> GHMSQSNRELVVDFLSYKLSQKGYSWSQFSDVEENRTEAPEETEAERETPSAINGNPSWHLADSPAVNGATGHSSSLDAREVIPESAVKQALREAGDEFELRYRRAFSDLTSQLHITPGTAYQSFEQVVNELFRDGVNWGRIVAFFSFGGALCVESVDKEMQVLVSRIASWMATYLNDHLEPWIQENGGWDTFVDLYG;> XIWIAQELRRRGDSFNAYYAR

Another subgroup is composed of antiapoptotic proteins, BCL-2, BCL-XL, BCl-w, MCL-1, A1 and BCL-B, which contain the BH1-BH4 domains that are arranged to form an extended hydrophobic groove known as the BH3-binding groove. The antiapoptotic BCL-2 subfamily proteins bind the BH3 domain of BAX/BAK and of the BH3-only proteins through their BH3-binding groove. Anticancer BH3 peptides have been developed, especially those derived from BIM, which interacts with all of the antiapoptotic proteins with extremely high affinity. Herein, we describe the embedment of the Akt recognition sequence into the BIM BH3 peptide and the cancer cell-specific apoptogenic property of the resulting BIM BH3 peptide variant characterized by X-ray crystallography, calorimetry and cell-based biochemistry.

To test if phosphorylated BH3BIM(I155R/E158S) binds to the BCL-2 family proteins more tightly than its unphosphorylated version, we produced recombinant BCL-2 and BCL-XL proteins, and also prepared two 21-mer synthetic peptides: BH3BIM(I155R/E158S) and phosphorylated BH3BIM(I155R/E158S) at Ser158, which is referred to as p-BH3BIM(I155R/E158S). Quantification of the binding affinities by isothermal titration calorimetry (ITC) showed that p-BH3BIM(I155R/E158S) interacted potently with BCL-2 and BCL-XL with KD values of 8.55 and 9.90 nM, respectively, similar to that of a longer 36-mer BIM BH3 peptide (KD of ~7 nM). To understand the structural basis for the critical role of the Ser158 phosphorylation, we next determined the crystal structure of BCL-XL bound to p-BH3BIM(I155R/E158S) at a 2.1-Å resolution. The peptide binds to the BH3-binding groove of BCL-XL by forming an amphipathic α-helix, as observed in all of the reported structures of the BH3 peptides bound to the antiapoptotic BCL-2 family proteins, 15, 31. The p-BH3BIM(I155R/E158S) peptide contains four of the five consensus residues that are highly conserved in the BH3 domains of the proapoptotic proteins and known to have critical roles in interacting with the antiapoptotic BCL-2 proteins. The four residues (Ile148, Leu152, Asp157 and Phe159) in the peptide are involved in the intermolecular hydrophobic or hydrophilic interactions with BCL-XL, similar to the corresponding residues of the BIML BH3 bound to BCL-XL (not shown). The remaining consensus residue, which corresponds to Ile155 of human BIM (Ile97 of mouse BIM), is replaced by arginine in p-BH3BIM(I155R/E158S). While Ile97 of mouse BIM is involved in hydrophobic interactions with Phe97 and Tyr101 of BCL-XL, Arg155 of p-BH3BIM(I155R/E158S) forms a hydrophobic interaction with Tyr101 through its hydrocarbon portion, and makes an intramolecular salt bridge with Glu151 of the peptide through its guanidinium group. The salt bridge is likely to increase the helical propensity of p-BH3BIM(I155R/E158S) in solution and to contribute to the binding affinity of this phosphorylated peptide.>MGAMIVKEVYETAEKIKSMEIRGAGRIARAAAQALMIQAEKSKAKEPEELWNELKVASKILYNTRPTAVSLPNALRYVMHRVKAAYLGGADLETLRFTAINSAKEFIYNSEKAIERIGEIGAKRIEDGDIIMTHSHSKAAISVMKKAFEQGKNIKVIVTETRPKWQGKITAKELASYGIPVIYIVDSAARHYMKMTDKVVMGADSITANGAVINKIGTSLIALTAKEHRVWVMIAAETYKFHPATMLGQLVEIEMRDPTEVIPEEELRTWPKNIEVWNPAFDVTPPEYIDVIITE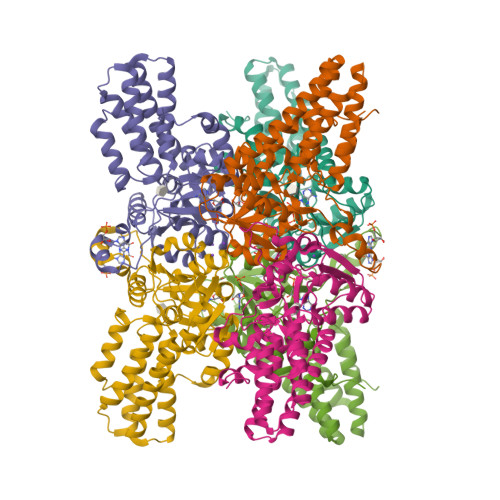RGIIPPYAAIDILKEEFGWALKYKEPWED[3x]8,9,10-TRIHYDROXY-7-HYDROXYMETHYL-3-METHYL-6-OXA-1,3-DIAZA-SPIRO[4.5]DECANE-2,4-DIONE | C9 H14 N2 O7 | 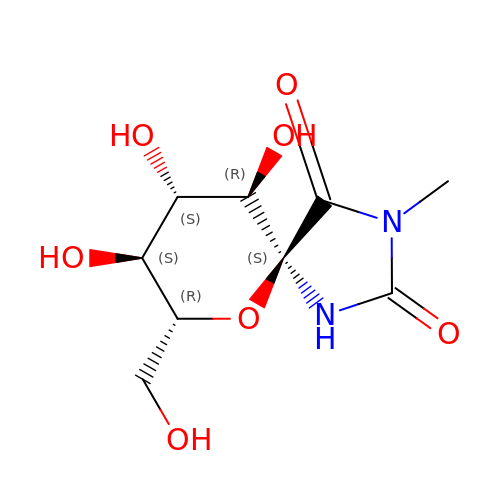RIUIMUSXAGXXON-FMTWGGRWSA-N> MTNSDDDLFSEKSTSSDTQQVQNILELEAKIPDILSSAGKCIEAIQLNNSLEDFRKYSKEFLETVEFISTGLRRQALELEKAEVPVVSLQPKKRYASTP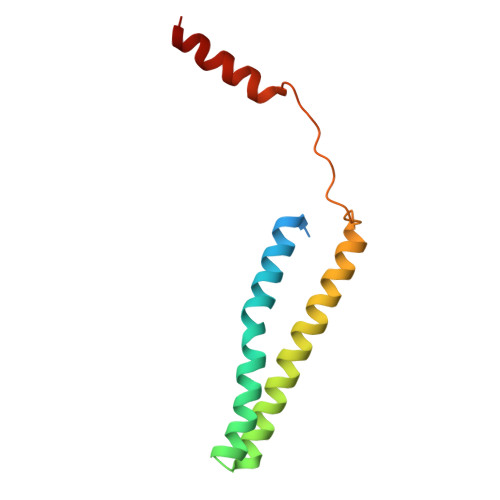LSNLIFDQSSKLM> HKCDITLQEIIKTLNSLTEQKTLCTELTVTDIFAASKNTTEKETFCRAATVLRQFYSHHEKDTRCLGATAQQFHRHKQLIRFLKRLDRNLWGLAGLNSCPVKEANQSTLENFLERLKTIMREKYSKCSS;> ADPFKVLQEPTCVSDYMSISTCEWKMNGPTQCSTELRLLYQLVFLLSEAHTCIPENNGGAGCVCHLLMDDVVSADQYTLDLWAGQQLLWKGSFKPSEHVKPRAPGNLTVHTQVSDTLLLTWSNPYPPDNYLYNHLT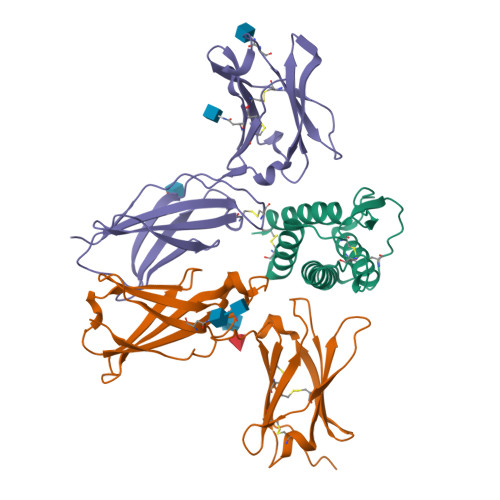YAVNIWSENDPADFRIYQVTYLEPSLRIAASTLKSGISYRARVRAWAQCYNTTWSEWSPSTKWHNSYRE;> PLPEVQCFVFNVEYMNCTWQSSSEPQPTNLTLHYWYKNSDNDKVQKCSHYLFSEEITSGCQLQKKEIHLYQTFVVQLQDPREPRRQATQMLKLQNLVIPWAPENLTLHKLSESQLELNWNNRFLNHCLEHLVQYRTDWDHSWTEQSVDYRHKFSLPSVDGQKRYTFRVRSRFNPLCGSAQHWSEWSHPIHWGSNTSKEN>[2x]SEKYFVKNGQPHFLISGEVHYFRINPKLWRNHLQLLKQTGADTVSTYIPWDWHEIEEDDFDFEGKTHPARNLIRFIKLCKEENLDLIVKPGPYILAEYENQGLPSWLLKKLSKNAFALDENGNVISPDLVSYLSDEFLEYTFKWYDKVMPIISKHQKEHYGPITMMQLCNEIGVFQWLSGKSDYNPKVINLYKEFIIQRYKTIEKLNSVYSTNYNSFDDLKAPSGKIKLRSDYCAYFDFHLFFREYYNKYISILKNKIRSFGINIKLTHNIPGWIYGNASELPMLISTYSEIMKNHPDIIFGLDHIPEFVSFRNAHSDLACNKILEAMQPEAPVWAAEFQAGTREHHVKAYAKDLETFYIASLAHGIKGFNYYMFSQGINPEGKGFYGKTFYFQTALDAASNKLALYDSIKKVNRFIRKEQKDLLRTNVNSEICVGFYKPYFFTELISSQLLKEKKLNVEELGLYIDPRFLREEILFNGLLRGLQTLNYNYDVVDLENCDLKSLTAYKQLWITSAEFMDAETQNLLSEFVLNGGNLILYPAVPTLDNYLNRCEILKNNFGIEFITKDSSHKVSAFGIEDVFTAFSKKQIYNDTNSKPIAFTQENEICGIRKKIGKGELTILGFAFGYTSDEHLELIDKLVKLNKIKRELFVSDKDIQFVVRENNKSRYIFFLNYHNERKTFNYRKSSELKKKKSEEISIAPFSYKVIKENK

The IALB_1185 protein, which is encoded in the gene cluster for endo-β-1,2-glucanase homologs in the genome of Ignavibacterium album, is a glycoside hydrolase family (GH) 35 protein. Here, we showed using recombinant IALB_1185 that this protein has glycosyltransferase activity toward β-1,2-glucooligosaccharides, and that the kinetic parameters for β-1,2-glucooligosaccharides are not within the ranges for general GH enzymes. Kinetic analysis further revealed that the enzyme has wide aglycone specificity regardless of the anomer, and that the β-1,2-linked glucose dimer sophorose is an appropriate donor. We propose that IALB_1185 be redefined β-1,2-glucooligosaccharide:d-glucoside β-d-glucosyltransferase as a systematic name and β-1,2-glucosyltransferase as an accepted name.

The overall conformational change on binding of ligands is small (rmsd, approximately 0.2 Å). Thus, the wild-type (WT)-Sop2 complex was used as a representative structure in Figure 3. The electron densities of Sop2 were clearly observed in both subunits of the WT-Sop2 complex. The fitted Sop2 molecules in subunits A and B are β- and α-anomers of Sop2, respectively. When the GlcN recognition residues in the TkGlmA-GlcN complex are aligned with the corresponding residues in the WT-Sop2 complex, the Glc moiety at the nonreducing end of Sop2 is well superimposed with the GlcN molecule, suggesting that Sop2 is bound at subsites −1 and +1. At subsite −1 in the WT-Sop2 complex, the distance between the carboxy group oxygen atom in the Glu343 side chain and the anomeric carbon atom (3.0 Å for both subunits) and the angle formed by the two atoms and the glycosidic bond oxygen atom in the Sop2 molecule (159° for subunit A and 165° for subunit B) are suitable for nucleophilic (in-line) attack on the anomeric center of the Glc moiety by Glu343. The carboxy group of the Glu176 side chain interacts with the scissile bond oxygen atom in the Sop2 molecule (2.6 Å between the two atoms) and is located where anti-protonation can occur. These results suggest that Glu343 and Glu176 are the nucleophile and acid/base, respectively. In the WT-Glc complex, Arg349 participates in substrate recognition to give a stable conformation, whereas Glu102 is still disordered or flips out as the ligand-free structure. Contrarily, in the WT-Sop2 complex, the Glu102 residue in each subunit clearly faces subsite −1 to form hydrogen bonds with the Glc moiety, suggesting that the side chain of Glu102 must interact with a Glc moiety at subsite −1 to face in the direction of subsite −1. In the complex of wild-type IALB_1185 with sophorose, the electron density of sophorose was clearly observed at subsites −1 and +1, whereas in the E343Q mutant–sophorose complex, the electron density of sophorose was clearly observed at subsites +1 and +2.~{N}-cycloheptyl-4-methyl-piperidine-1-carboxamide | 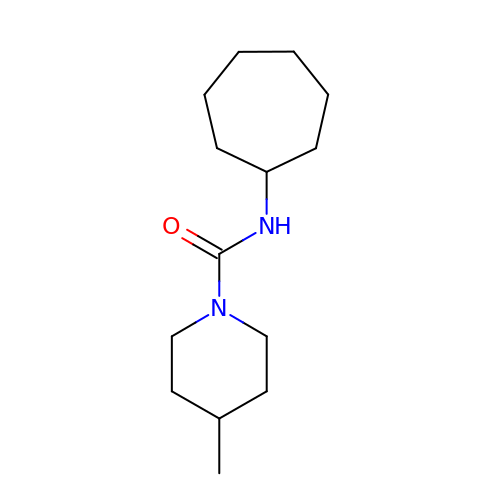C14 H26 N2 O | RBBIAFZDUSBCMN-UHFFFAOYSA-N>TEEQKQEIREAFDLFDADGTGTIDVKELKVAMRALGFEPKKEEIKKMISEIDKEGTGKMNFGDFLTVMTQKMSEKDTKEEILKAFKLFDDDETGKISFKNLKRVAKELGENLTDEELQEMIDEADRDGDGE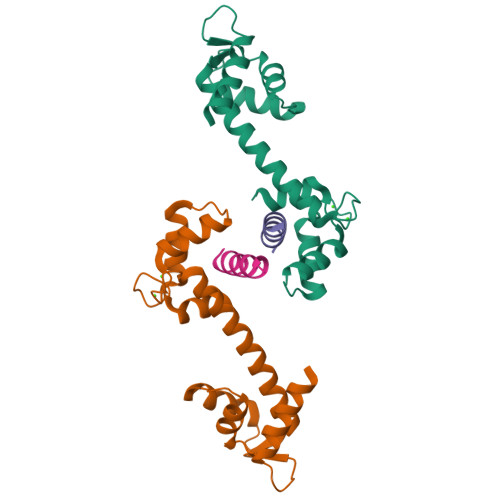VSEQEFLRIMKK[2x];>[2x]XNWKLLAKGLLIRERLKR>MWLRLGPPSLSLSPKPTVGRSLCLTLWFLSLALRASTQAPAPTVNTHFGKLRGARVPLPSEILGPVDQYLGVPYAAPPIGEKRFLPPEPPPSWSGIRNATHFPPVCPQNIHTAVPEVMLPVWFTANLDIVATYIQEPNEDCLYLNVYVPTEDVKRISKECARKPNKKICRKGGSGAKKQGEDLADNDGDEDEDIRDSGAKPVMVYIHGGSYMEGTGNMIDGSILASYGNVIVITLNYRVGVLGFLSTGDQAAKGNYGLLDQIQALRWVSENIAFFGGDPRRITVFGSGIGASCVSLLTLSHHSEGLFQRAIIQSGSALSSWAVNYQPVKYTSLLADKVGCNVLDTVDMVDCLRQKSAKELVEQDIQPARYHVAFGPVIDGDVIPDDPEILMEQG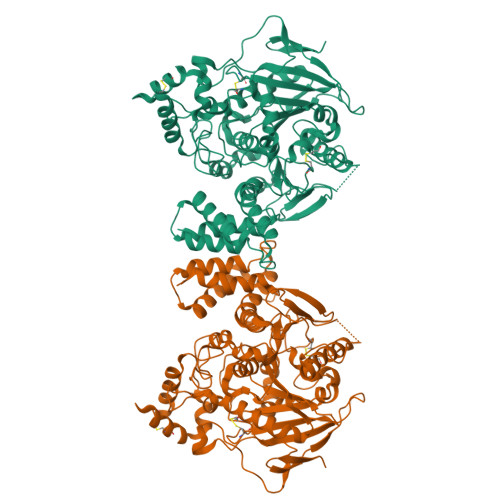EFLNYDIMLGVNQGEGLKFVEGVVDPEDGVSGTDFDYSVSNFVDNLYGYPEGKDTLRETIKFMYTDWADRDNPETRRKTLVALFTDHQWVEPSVVTADLHARYGSPTYFYAFYHHCQSLMKPAWSDAAHGDEVPYVFGVPMVGPTDLFPCNFSKNDVMLSAVVMTYWTNFAKTGDPNKPVPQDTKFIHTKANRFEEVAWSKYNPRDQLYLHIGLKPRVRDHYRATKVAFWKHLVPHLYNLHDMFHYTSTTTKVPPPDTTHSSHITRRPNGKTWSTKRPAISPAYSNENAQGSWNGDQDAGPLLVENPRDYSTELSVTIAVGASLLFLNVLAFAALYYRKDKRRQEPLRQPSPQRGAGAPELGAAPEEELAALQLGPTHHECEAGPPHDTLRLTALPDYTLTLRRSPDDIPLMTPNTITMIPNSLVGLQTLHPYNTFAAGFNSTGLPHSHSTTRV[2x]>CUGCUGCUGCUGCUGCUG[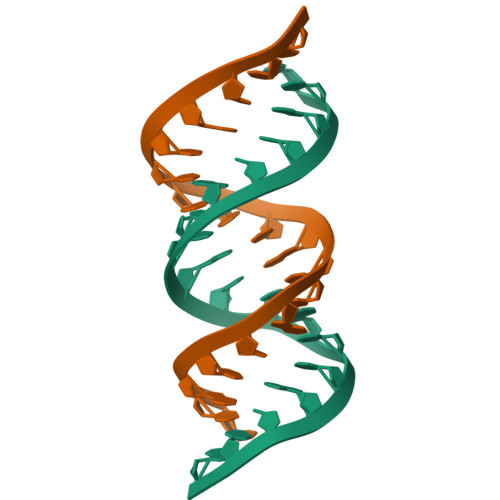2x]> MGHHHHHHARSVRHIAIPAHRGLITDRNGEPLAVSTPVTTLWANPKELMTAKERWPQLAAALGQDTKLFADRIEQNAEREFIYLVRGLTPEQGEGVIALKVPGVYSIEEFRRFYPAGEVVAHAVGFTDVDDRGREGIELAFDEWLAGVPGKRQVLKDRRGRVIKDVQVTKNAKPGKTLALSIDLRLQYLAHRELRNALLENGAKAGSLVIMDVKTGEILAMTNQPTYNPNNRRNLQPAAMRNRAMIDVFEPGSTVKPFSMSAALASGRWKPSDIVDVYPGTLQIGRYTI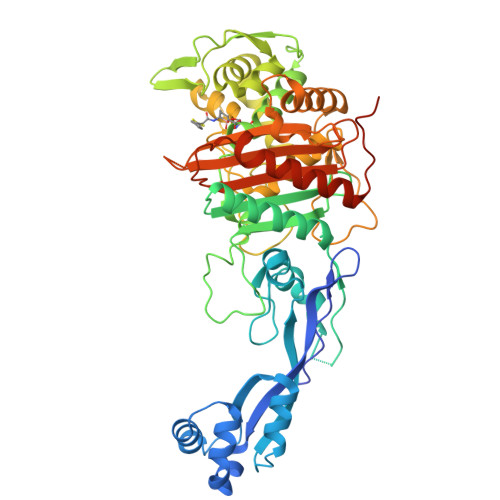RDVSRNSRQLDLTGILIKSSNVGISKIAFDIGAESIYSVMQQVGLGQDTGLGFPGERVGNLPNHRKWPKAETATLAYGYGLSVTAIQLAHAYAALANDGKSVPLSMTRVDRVPDGVQVISPEVASTVQGMLQQVVEAQGGVFRAQVPGYHAAGKSGTARKVSVGTKGYRENAYRSLFAGFAPATDPRIAMVVVIDEPSKAGYFGGLVSAPVFSKVMAGALRLMNVPPDNLPTATEQQQVNAAPAKGGRG> MSSVFDEYEQLLAAQTRPNGALGGGEKGSTLKVEVPVFTLNSDDPEDRWNFAVFCLRIAVSEDANKPLRQGALISLLCSHSQVMRNHVALAGKQNEATLAVLEIDGFTNGVPQFNNRSGVSEERAQRFMMIAGSLPRACSNGTPFVTAGVEDDAPEDITDTLERILSIQAQVWVTVAKAMTAYETADESETRRINKYMQQGRVQKKYILHPVCRSAIQLTIRQSLAVRIFLVSELKRGRNTAGGTSTYYNLVGDVDSYIRNTGLTAFFLTLKYGINTKTSALALSSLSGDIQKMKQLMRLYRMKGDNAPYMTLLGDSDQMSFAPAEYAQLYSFAMGMASVLDKGTGKYQFARDFMSTSFWRLGVEYAQAQGSSINEDMAAELKLTPAARRGLAAAAQR

One remarkable character of negative-strand RNA viruses is that their genomes are enwrapped by the nucleoprotein (N), which results in the formation of helical nucleocapsids. N has two domains, the amino-terminal domain (NTD) and the carboxy-terminal domain (CTD), with a positively charged cleft in between that is suitable for RNA binding. In the presence of RNA, each N can bind 6, 7 or 9 nucleotides and thus can clamp RNA into the cleft, forming a ribonucleoprotein complex (RNP). Here, the Newcastle disease virus (NDV), a member of the genus Avulavirus, family Paramyxoviridae, which is relatively safe for handling, was selected as the model to look at how NDV RNP protects its viral genome and to provide new insights into the development of nucleocapsid-based antivirus therapies.

Different from the reported ring-structure and helical spirals, a novel clam-shaped structure of NDV N with two single-turn spirals packing in a back-to-back manner was identified and determined, corresponding to the extracted nucleocapsid assembly of NDV. Further 3D refinement resolved the clam-shaped structure to 6.4 Å resolution and showed obvious C2 symmetry in the rigid body. The C2 symmetry was then applied to improve the resolution, yielding an overall 4.8 Å resolution of the core structure. Homolog modeling on NDV N, based on the 40% sequence identity of N between NDV and Parainfluenza virus 5 (PIV5), resulted the subunit N model and the model was flexibly docked into the EM density map. The docked model fits the EM density well with only minor modification, and resulted in a reliable initial model of NDV N. In the clam-shaped structure or in the derived double-headed filament, the self-capping interface came from loops (residues 114–120) of vertically adjacent N in the clam-shaped core. Distance analysis of the residues in the loop suggested that hydrogen bonds may exist between two pairs of Glysin119 and Arginine117 residues. The evidence suggests that Loop114–120 has no influence on helical assembly but has a crucial role in clam-shaped structure formation. The double-headed spiral uses a self-capping mechanism that involves the clam-shaped core to protect the RNA genome’s integrity. The C-tail is located inside the clam-shaped structure, and is only accessible from either end by P or other proteins in order to form the N–RNA–RdRp complex for the replication and transcription of the genomic RNA; this finding differs from those of previous reports that have described outside-orientated C-tails.>[6x]GHHHHHHELANNTTGFTRIIKAAGYSWKGLRAAWINEAAFRQEGVAVLLCVVIAAWLDVDAVTRVLLISSVMLVMIVELLNSAIEAVV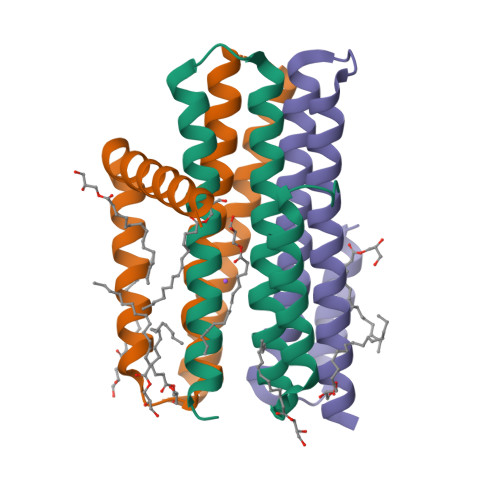DRIGSEYHELSGRAKDLGSAAVLIAIIDAVITWAILLWSHFG>MQQLNENKIIKLLRDNIPKLQLIYLFGSYSQGTQHRNSDIDIAVLAADTLDNIARWELAQKLASALDSDVDLVDLRSASTVLCQQVVTQGKQLWGTQQDDELFAVKTIS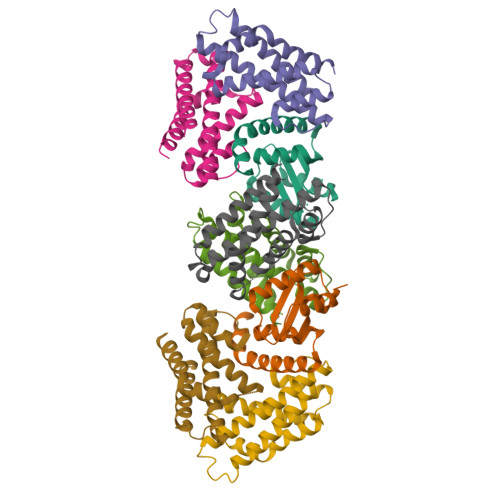MYQHLQAERQAIIDDVMANTAAKAHRGESL[2x];>MNDIIINKIATIKRCIKRIQQVYGDGSQFKQDFTLQDSVILNLQRCCEACIDIANHINRQQQLGIPQSSRDSFTLLAQNNLITQPLSDNLKKMVGLRNIAVHDAQELNLDIVVHVVQHHLEDFEQFIDVIKAE[6x]5'-O-[(R)-(cyclopropyloxy)(hydroxy)phosphoryl]adenosine 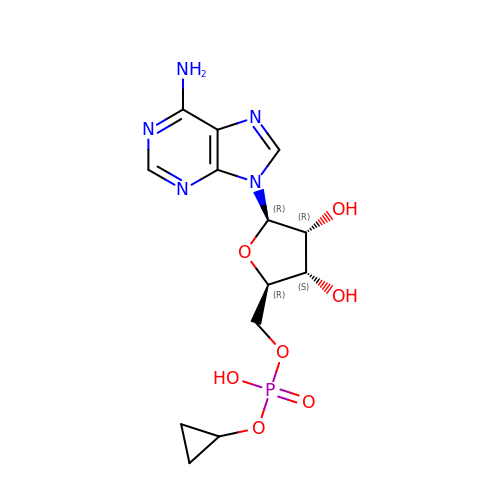| C13 H18 N5 O7 P | FJCZQSQASCNEEZ-QYVSTXNMSA-N>MASMYNSDGWYMGEAINMASLNTCAADLGKWQNFIDDYTSNDYYKGTPYIDWVFASSPKGDRWQMNEWSVSEMLKVGGTYEEGGLNCMGFVWHAIAKGLSVESGLDISQTGQYVPFSSYFNGLGLSRKCWATPGGSGGWTVFVDYYNLHYYEFPTKEEMLSSGVLQKGD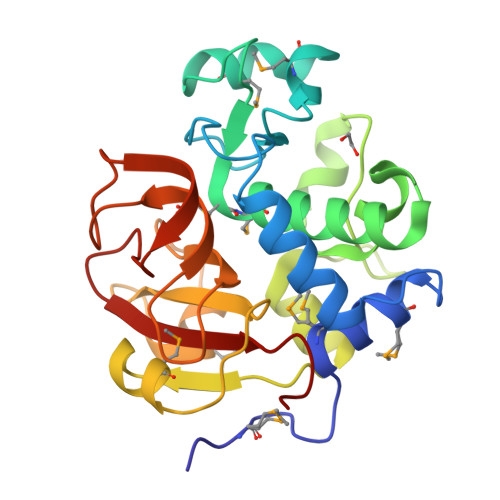IIWCVDGSVGLGMAGLRTIADNHHIGIYTGNGTSDSWWQSGPVKADGDLVNVGTDVCPIYGAAAKNTYVVLPWAKKA[2x]>DRHHHHHHKLSPPAAPRFNVSLDSVPELRWLPVLRHYDLDLVRAAMAQVIGDRVPKWVHVLIGKVVLELERFLPQPFTGEIRGMCDFMNLSLADALLVNLAYESSVFATSIVAQDSRGHIYHGRNLDYPFGNVLRKLTVDVQFLKNGQIAFTGTTFIGYV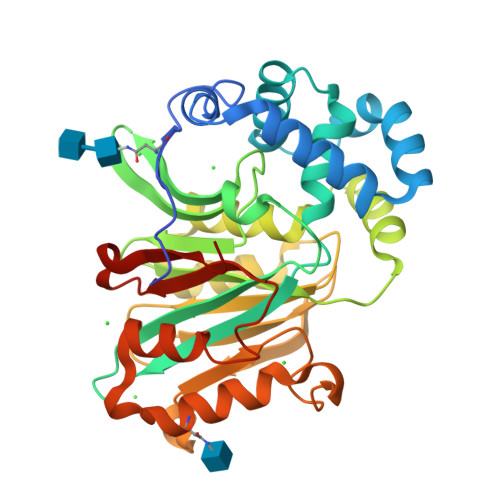GLWTGQSPHKFTVSGDERDKGWWWENAIAALFRRHIPVSWLIRATLSESENFEAAVGKLAKTPLIADVYYIVGGTSPREGVVITRNRDGPADIWPLDPLNGAWFRVETNYDHWKPAPKEDDRRTSAIKALNATGQANLSLEALFQILSVVPVYNNFTIYTTVMSAGSPDKYMTRIRNPSRK[4x]> MRQVWFSWIVGLFLCFFNVSSAAQYEPPATWENVDYKRTIDVSNAYISETIEITIKNIASEPATEYFTAFESGIFSKVSFFSAYFTNEATFLNSQLLANSTTAPGDDGESEIRYGIIQFPNAISPQEEVSLVIKSFYNTVGIPYPEHVGMSEEQHLLWETNRLPLSAYDTKKASFTLIGSSSFEEYHPPNDESLLGKANGNSFEFGPWEDIPRFSSNETLAIVYSHNAPLNQVVNLRRDIWLSHWASTIQFEEYYELTNKAAKLSKGFSRLELMKQIQTQNMRQTHFVTVLDMLLPEGATDHYFTDLVGLVSTSHAERDHFFIRPRFPIFGGWNYNFTVGWTNKLSDFLHVSSGSDEKFVASIPILNGPPDTVYDNVELSVFLPEGAEIFDIDSPVPFTNVSIETQKSYFDLNKGHVKLTFSYRNLISQVANGQVLIKYDYPKSSFFKKPLSIACYIFTALMGVFVLKTLNMNVTN;> MAKAPKANTPKVTSTSSAVLTDFQETFKTSKRAYFAQIEKYPKLKLI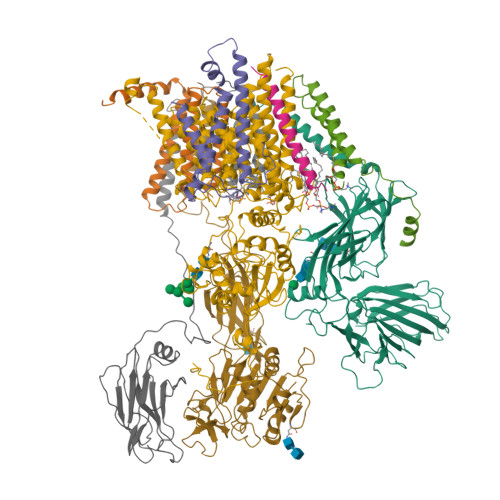DTFCFFLVLLGVIQCTFIILIRDNFPFNAFLAGFIICVGQFVLLMSLRLQLCNSFPGISKNRAFAEFIVASLILHFVCLHFIN;> MNWLFLVSLVFFCGVSTHPALAMSSNRLLKLANKSPKKIIPLKDSSFENILAPPHENAYIVALFTATAPEIGCSLCLELESEYDTIVASWFDDHPDAKSSNSDTSIFFTKVNLEDPSKTIPKAFQFFQLNNVPRLFIFKPNSPSILDHSVISISTDTGSERMKQIIQAIKQFSQVNDFSLHLPMDWTPIITSTIITFITVLLFKKQSKLMFSIISSRIIWATLSTFFIICMISAYMFNQIRNTQLAGVGPKGEVMYFLPNEFQHQFAIETQVMVLIYGTLAALVVVLVKGIQFLRSHLYPETKKAYFIDAILASFCALFIYVFFAALTTVFTIKSPAYPFPLLRLSAPFK;> MISDEQLNSLAITFGIVMMTLIVIYHAVDSTMSPKN;> MTYEQLYKEFHSSKSFQPFIHLDTQPKFAICGLIVTLAVLSSALFAVGSKSSYIKKLFFYTILSVIGSLFAGLTTVFASNSFGVYV;> MGSDRSCVLSVFQTILKLVIFVAIFGAAISSRLFAVIKFESIIHEFDPWFNYRATKYLVNNSFYKFLNWFDDRTWYPLGRVTGGTLYPGLMTTSAFIWHALRNWLGLPIDIRNVCVLFAPLFSGVTAWATYEFTKEIKDASAGLLAAGFIAIVPGYISRSVAGSYDNEAIAITLLMVTFMFWIKAQKTGSIMHATCAALFYFYMVSAWGGYVFITNLIPLHVFLLILMGRYSSKLYSAYTTWYAIGTVASMQIPFVGFLPIRSNDHMAALGVFGLIQIVAFGDFVKGQISTAKFKVIMMVSLFLILVLGVVGLSALTYMGLIAPWTGRFYSLWDTNYAKIHIPIIASVSEHQPVSWPAFFFDTHFLIWLFPAGVFLLFLDLKDEHVFVIAYSVLCSYFAGVMVRLMLTLTPVICVSAAVALSKIFDIYLDFKTSDRKYAIKPAALLAKLIVSGSFIFYLYLFVFHSTWVTRTAYSSPSVVLPSQTPDGKLALIDDFREAYYWLRMNSDEDSKVAAWWDYGYQIGGMADRTTLVDNNTWNNTHIAIVGKAMASPEEKSYEILKEHDVDYVLVIFGGLIGFGGDDINKFLWMIRISEGIWPEEIKERDFYTAEGEYRVDARASETMRNSLLYKMSYKDFPQLFNGGQATDRVRQQMITPLDVPPLDYFDEVFTSENWMVRIYQLKKDDAQGRTLRDVGELTRSSTKTRRSIKRPELGLRV;> MRTDWNFFFCILLQAIFVVGTQTSRTLVLYDQSTEPLEEYSVYLKDLEQRNYKLEYLDINSTSTTVDLYDKEQRLFDNIIVFPTKGGKNLARQIPVKQLIKFFENEGNILCMSSPGAVPNTIRLFLNELGIYPSPKGHVIRDYFSPSSEELVVSSNHLLNKYVYNARKSEDFVFGESSAALLENREQIVPILNAPRTSFTESKGKCNSWTSGSQGFLVVGFQNLNNARLVWIGSSDFLKNKNQDSNQEFAKELLKWTFNEKSVIKSVHAVHSHADGTSYDEEPYKIKDKVIYSVGFSEWNGEEWLPHIADDIQFELRQVDPYYRLTLSPSGNDSETQYYTTGEFILPDRHGVFTFLTDYRKIGLSFTTDKDVKAIRHLANDEYPRSWEISNSWVYISAICGVIVAWIFFVVSFVTTSSVGKKLETFKKTN;> MQFFKTLAALVSCISFVLAYVAQDVHVSFPSTAGKSRVMIGKVEPRIGIDETVPTTITVEDPNEVIQVNFAIESTNKPFQNTLLIGLPNKNLEMAFEPEIKDNGKLSMYKYRIDLAKLDAALLQEASRSPEPIKATLILASSTAKPKENLFREILQLNLNFDVDHSDSSLVDKFGIKPEIHHIFHAEPKRVAKPIAVIFVLIIFITILSLIVTWLNSCAAAFNNIPTGVTAVYFLGFIATIVGFEVIFARYYLGTSIFETLFSSLYLGAPGLLTSTKFLRSFGQTI N-(4-methylpentanoyl)-L-phenylalanine 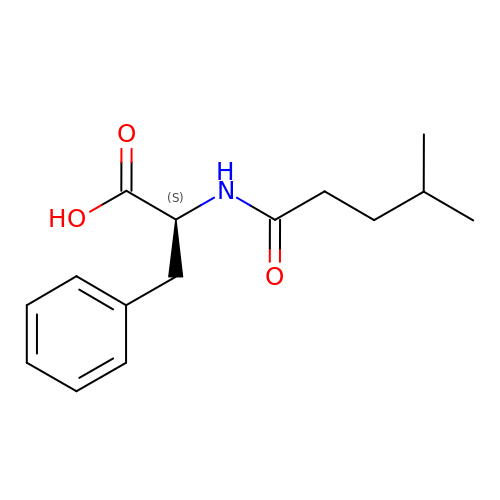| C15 H21 N O3 | SNFOUMUDOQSPKF-ZDUSSCGKSA-N>[3x]GIEDLIDTAIKNALRVSQPPSTQSTEATSGVNSQEVPALTAVETGASGQAIPSDVVETRHVVNYKTRSESCLESFFGRAACVTILSLTNSSKSGEEKKHFNIWNITYTDTVQLRRKLEFFTYSRFDLEMTFVFTENYPSTASGEVRNQVYQIMYIPPGAPRPSSWDDYTWQSSSNPSIFYMYGNAPPRMSIPYVGIANAYSHFYDGFARVPLEGENTDAGDTFYGLVSINDFGVLAVRAVNRSNPHTIHTSVRVYMKPKHIRCWCPRPPRAVLYRGEGVDMISSAILPLAKVDSITTF;>[3x]SPNVEACGYSDRVRQITLGNSTITTQEAANAIVAYGEWPTYINDSEANPVDAPTEPDVSSNRFYTLESVSWKTTSRGWWWKLPDCLKDMGMFGQNMYYHYLGRSGYTIHVQCNASKFHQGALGVFLIPEFVMACNTESKTSYVSYINANPGERGGEFTNTYNPSNTDASEGRKFAALDYLLGSGVLAGNAFVYPHQIINLRTNNSATIVVPYVNSLVIDCMAKHNNWGIVILPLAPLAFAATSSPQVPITVTIAPMCTEFNGLRNITVPVHQ;>[3x]GLPTMNTPGSNQFLTSDDFQSPCALPNFDVTPPIHIPGEVKNMMELAEIDTLIPMNAVDGKVNTMEMYQIPLNDNLSKAPIFCLSLSPASDKRLSHTMLGEILNYYTHWTGSIRFTFLFCGSMMATGKLLLSYSPPGAKPPTNRKDAMLGTHIIWDLGLQSSCSMVAPWISNTVYRRCARDDFTEGGFITCFYQTRIVVPASTPTSMFMLGFVSACPDFSVRLLRDTPHISQSKLIGRTQ;>[3x]MGAQVSTQKTGAHENQNVAANGSTINYTTINYYKDSASNSATRQDLSQDPSKFTEPVKDLMLKTAPALN

Non-polio enteroviruses (NPEVs) from the family of Picornaviridae are nonenveloped viruses composed of (+) ssRNA genomes that infect humans and cause a variety of human diseases. For this proof-of-concept study, we selected CV-A21 viral strain responsible for a substantial proportion of enterovirus-associated acute respiratory tract infections in humans. Herein, we introduce an EMPEM pipeline for rapid structural analysis of pAb responses elicited by enteroviruses using whole viral particles. Using a combination of nsEM- and cryoEM-based polyclonal epitope mapping, we identified two primary immunogenic sites on the surface of CV-A21 located near the 3-fold and 5-fold axes.

Through iterative rounds of focused classification, we reconstructed maps featuring structurally distinct polyclonal antibodies bound to epitopes at near-atomic resolution (structurally distinct polyclonal antibody class—pAbC). We resolved two distinct polyclonal antibodies targeting Site-1 and three against Site-2. The highest achieved global map resolution was 3.8 Å (pAbC1-1), although the local resolution was worse for the pAb-corresponding part of the map. We next relaxed atomic models into the pAbC1-1, pAbC2-1, and pAbC2-3 cryoEMPEM maps. Given the polyclonal nature of bound antibodies and the inherent lack of sequence information, the variable Fab domains (Fv) were represented as poly-Alanine models. Specific epitope contacts and angle of approach were highly similar for Site-1 antibodies while Site-2 pAbs displayed greater diversity; consistent with nsEM analysis. CryoEMPEM maps and corresponding models were used to assign specific epitope contacts for Site-1 and Site-2 pAbs. While antibodies targeting Site-1 are distal from the RBS and it is unlikely that they would interfere with receptor binding as Fabs, antibodies against Site-2 sterically block ICAM-1 from accessing the RBS and may be able to suppress viral entry. Overall, we observed a high degree of similarity in epitopes for several of the antibodies. For example, Site-1 overlaps with the binding sites of 14B10 (15), 5F5 (16), and 2G8 (26) mAbs; the overlay of pAbC1-1 and 14B10 mAb structures is shown in the Supplementary Material Appendix—Fig. S7A. Importantly, all pAbs bind in a manner that does not block the accessibility to the symmetry-related neighboring binding site.> IWELKKDVYVVELDWYPDAPGEMVVLTCDTPEEDGITWTLDQSSEVLGSGKTLTIQVKEFGDAGQYTCHKGGEVLSHSLLLLHKKEDGIWSTDILKDQKEPKNKTFLRCEAKNYSGRFTCWWLTTISTDLTFSVKSSRGSSDPQGVTCGAATLSAERVRGDNKEYEYSVECQEDSACPAAEESLPIEVMVDAVHKLKYENYTSSFFIRDIIKPDPPKNLQLKPLKNSRQVEVSWEYPDTWSTPHSYFSLTFCVQVQGKSKREKKDRVFTDKTSATVICRKNASISVRAQDRYYSSSWSEWASVPCS;> RAVPGGSSPAWTQCQQLSQKLCTLAWSAHPLVGHMDLREEGDEETTNDVPHIQCGDGCDPQGLRDNSQFCLQRIHQGLIFYEKLLGSDIFTGEPSLLPDSPVGQLHASLLGLSQLLQPEGHHWETQQIPSLSPSQPWQRLLLRFKILRSLQAFVAVAARVFAHGAATLSPGTKHHHHHH;> HMSIQEIQKEIAQIQAVIAGIQKYIYTMTGGSGGSGGGGSGGSGGMSIEEIQKQIAAIQCQIAAIQKQIYAMTGSGGGGSGGSGGGGSGMSIEEIQKQIAAIQEQILAIYKQIMAMVT

The Alphabody scaffold is a computationally designed protein scaffold of about 10 kDa molecular weight, which was developed to serve as a therapeutic agent. The scaffold does not have a counterpart in nature and is composed of a single contiguous polypeptide chain designed to adopt a triple-helix coiled-coil fold. IL-23 adopts an atypical heterodimeric structure consisting of a p40 subunit encompassing three fibronectin-III-like domains, which is linked via a disulfide bond to an α-helical bundle subunit (p19) that topologically resembles long-chain helical cytokines. We show that affinity-matured Alphabodies can bind with ultra-high affinity to IL-23, but not IL-12, via an extensive interaction interface that engages the p19 subunit of IL-23 to abrogate IL-23-mediated signalling in vitro and in vivo.

Crystallization trials of highly monodisperse preparations of the IL-23:MA12 complex yielded two distinct crystal forms that allowed us to determine crystal structures at 1.74 and 3.4 Å resolution, providing the opportunity to visualize the binding epitope in detail and to cross-validate structural observations. MA12 folds into a left-handed triple-helix coiled-coil structure, with the binding surface located mainly at the C-terminal half of helices A and C. In agreement with the ITC-derived stoichiometry of the complex, one copy of MA12 binds to the p19 subunit of IL-23 and is oriented parallel to the longitudinal axis of the p40 subunit. The respective binding interfaces feature 20 amino-acid residues contributed by MA12 and 28 amino-acid residues contributed by p19, burying a total surface area of 800 and 840 Å2, respectively. Five hydrogen bonds and two salt bridges are formed upon binding, while the rest of the interaction interface can be described in terms of van der Waals contacts. The binding interface is further hallmarked at its two ends by two prominent attachment points. At the other end, Tyr110 on MA12, a conserved residue in all matured binders, inserts into a pocket on IL-23 p19 defined by the BC and AB loops and the N-terminal part of helix D. Furthermore, we note that this segment of the AB loop in the p19 subunit of IL-23 is disordered in all currently available crystal structures of IL-23, suggesting that the interaction with the Alphabody induces the observed conformation. We were intrigued by persisting residual difference electron density emanating from the Cδ1 position of Trp319 in IL-23 p40 up to the last rounds of refinement. Indeed, mass spectrometry on tryptic peptides of our recombinant human IL-23 confirmed that Trp319 in the p40 subunit of IL-23 is mannosylated.>[2x]GPLGSDEGVVKEIPITHHVKEGYEKADPAQFELLKVLGQGSFGKVFLVRKKTGPDAGQLYAMKVLKKASLKVRDRVRTKMERDILVEVNHPFIVKLHYAFQTEGKLYLILDFLRGGDVFTRLSKEVLFTEEDVKFYLAELALALDHLHQLGI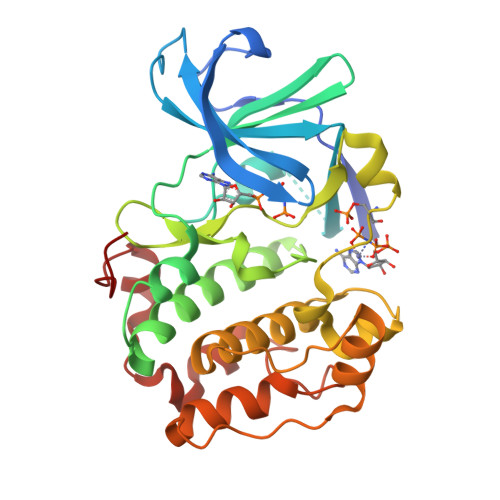VYRDLKPENILLDEIGHIKLTDFGLSKESVDQEKKAYSFCGTVEYMAPEVVNRRGHSQSADWWSYGVLMFEMLTGTLPFQGKDRNETMNMILKAKLGMPQFLSAEAQSLLRMLFKRNPANRLGSEGVEEIKRHLFFANIDWDKLYKREVQPPFKP>[2x]MALSAEGSSGGSRGGSPKAEAASVPSWPQILGRLTDNRDLARGQAAWAMDQIMTGNARPAQIAAFAVAMTMKAPTADEVGELAGVMLSHAHPLPADTVPDDAVDVVGTGGDGVNTVNLSTMAAIVVAAAGVPVVKHGNRAASSLSGGADTLEALGVRIDLGPDLVARSLAEVGIGFCFAPRFHPSYRHAAAVRAEIGVPTVFNLLGPLTNPARPRAGLIGCAFADLAEVMA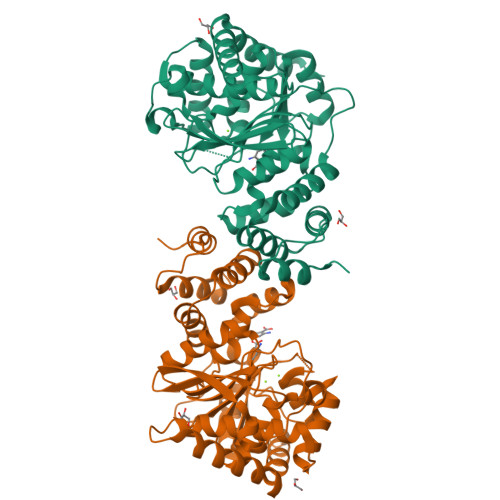GVFAARRSSVLVVHGDDGLDELTTTTTSTIWRVAAGSVDKLTFDPAGFGFARAQLDQLAGGDAQANAAAVRAVLGGARGPVRDAVVLNAAGAIVAHAGLSSRAEWLPAWEEGLRRASAAIDTGAAEQLLARWVRFGRQILEHHHHHH>ADDELYRQSLEIISRYLREQATGAKDTKP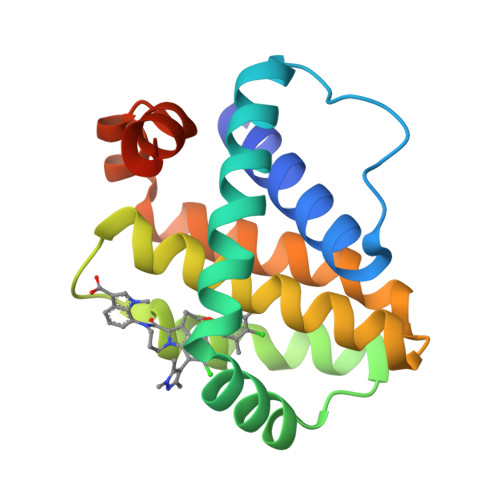MGRSGATSRKALETLRRVGDGVQRNHETAFQGMLRKLDIKNEDDVKSLSRVMIHVFSDGVTNWGRIVTLISFGAFVAKHLKTINQESCIEPLAESITDVLVRTKRDWLVKQRGWDGFVEFFHVEDLEGG[4x]> GSMTEIALIGNPNSGKTSLFNLITGHNQRVGNWPGVTVERKSGLVKKNKDLEIQDLPGIYSMSPYSPEEKVARDYLLSQRADSILNVVDATNLERNLYLTTQLIETGIPVTIALNMIDVLDGQGKKINVDKLSYHLGVPVVATSALKQTGVDQVVKKAAHTTTSTVGDLAFPIYDDRLEAAISQILEVLGNSVPQRSARFYAIKLF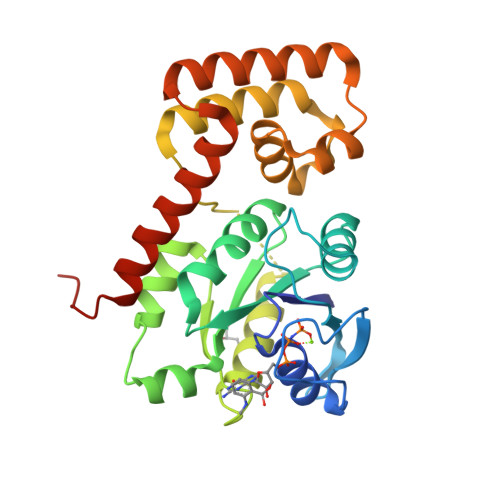EQDSLVEAELDLSQFQRKEIEDIIRITEEIFTEDAESIVINERYAFIERVCQMAESHTEDFALTLS>MEMGRRIHLELRNRTPSDVKELVLDNSRSNEGKLEGLTDEFEELE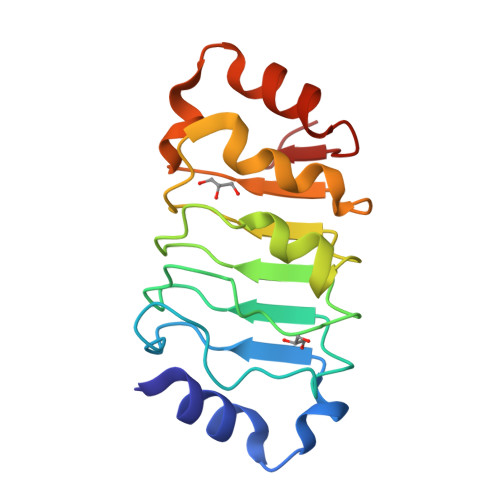FLSTINVGLTSIANLPKLNKLKKLELSDNRVSGGLEVLAEKCPNLTHLNLSGNKIKDLSTIEPLKKLENLKSLDLFNCEVTNLNDYRENVFKLLPQLTYLDGYD[6x]> GPLQDPQIKRQKMIYHCKFGEFGVMEGQFTEPSGVAVNAQNDIIVADTNNHRIQIFDKEGRFKFQFGECGKRDSQLLYPNRVAVVRNSGDIIVTERSPTHQIQIYNQYGQFVRKFGATILQHPRGVTVDNKGRIIVVECKVMRVIIFDQNGNVLHKFGCSKHLEFPNGVVVNDKQEIFISD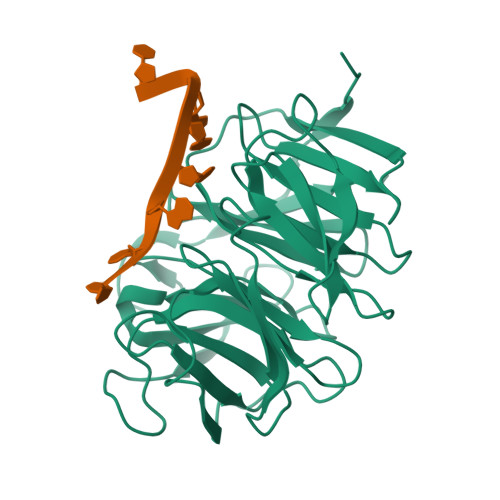NRAHCVKVFNYEGQYLRQIGGEGITNYPIGVGINSNGEILIADNHNNFNLTIFTQDGQLISALESKVKHAQCFDVALMDDGSVVLASKDYRLYIYRYVQLAPVGM Caspases are cysteine-dependent aspartyl-specific proteases involved in a range of cellular and disease processes, ranging from apoptosis to inflammation and neurodegeneration. Caspase family members are broadly classified as inflammatory (C1, C4, and C5) or apoptotic caspases. While often classified as an executioner caspase, the function of caspase-6 (C6) in physiology and disease has remained enigmatic, and it has been suggested that C6 may act upstream of the other executioner caspases. C6 possesses a non-catalytic cysteine (C264) not present in other family members and is situated on a loop in the small subunit at the distal end of the active site. The catalytic cysteine (C163) is found on the large subunit, while two additional cysteine residues appear to be buried and thus inaccessible for disulfide formation.

When tested in a biochemical assay, enantiomer 3a potently inhibited C6 activity with an IC50 value of 8 nM, while its enantiomer 3b exhibited an IC50 at least 100-fold weaker. A complex X-ray crystal structure of 3a showed similarities and differences as compared to the binding of 2a. Both analogues engaged C264 in a covalent bond as expected, while the trifluoromethoxyaryl side chain of both analogues was buried in the S1 pocket, where the aspartic acid residue of the C6 substrate is usually bound. To accommodate this large and hydrophobic ring system in S1, arginine 220, which formed hydrogen bonds with the aspartic acid in VEID peptide-type inhibitors, is moved by 4.2 Å (ε nitrogen) to create a hydrophobic cavity complementary in shape to the sidechain of 3a. However, the location and orientation of the piperidine ring and sulfonamide function were quite different in the two analogues. The phenyl substituent present in 3a made few, if any, contacts with the protein, but by occupying an equatorial position in the bound conformation, it energetically stabilized the required axial orientation of the trifluoromethoxy benzamide side chain of 3a, as bound in the S1 pocket. The potent low-nM inhibition of C6 WT protein by 3a was completely lost with the C264A mutant, further establishing that 3a engages C264. The potency and exquisite isoform selectivity of 3a, together with the lack of C6 activity for its enantiomer 3b, strongly suggested that 3a inhibits C6 by first forming a pre-covalent complex that positioned the electrophilic vinylsulfonamide for subsequent reaction with C264. To better understand C6 inhibition by 3a, we determined kinetic parameters (kinact/Ki values) of inhibition. These data indicated that indeed, both noncovalent and covalent interactions contributed to the binding, with a Ki value of 7.0 μM, providing an estimate of the intrinsic pre-covalent binding affinity of 3a for C6. None of the remaining seven putative off-target proteins were proteases; all are membrane-associated proteins, including two heme proteins (CYB5B and HMOX2) and one cysteine-dependent enzyme (PTGES2).

>[4x]MFDPAEKYKMDHRRRGIALIFNHERFFWHLTLPERRGTCADRDNLTRRFSDLGFEVKCFNDLKAEELLLKIHEVSTVSHADADCFVCVFLSHGEGNHIYAYDAKIEIQTLTGLFKGDKCHSLVGKPKIFIIQACRGNQHDVPVIPLDVVD;>[4x]MAASVYTLPAGADFLMCYSVAEGYYSHRETVNGSWYIQDLCEMLGKYGSSLEFTELLTLVNRKVSQRRVDFCKDPSAIGKKQVPCFASMLTKKLHFFPKSNLEHHHHHH Rhomboid intramembrane proteases are evolutionarily conserved proteins with numerous important biological functions, including growth factor secretion, regulation of mitochondrial dynamics, and membrane protein quality control (Fleig et al., 2012). Rhomboids are serine proteases with a Ser-His catalytic dyad (Wang et al., 2006), and they recognize their transmembrane substrates in a two-tier process. It is assumed that first a portion of the transmembrane domain of the substrate docks into an intramembrane interaction site of rhomboid within the plane of the lipid bilayer, upon which a linear segment of the substrate (possibly generated by local unfolding of the top of the substrate's transmembrane helix) interacts with the water-exposed active site (reviewed in Strisovsky, 2016a, Strisovsky, 2013).

To understand why peptidyl ketoamides are such efficient rhomboid inhibitors and to establish the basis for structure-guided design of their improved variants, we determined the co-crystal structures of GlpG with 9 and 10. The complexes were formed by soaking the inhibitors into apoenzyme crystals, and the structures were solved using diffraction data to 2.16 and 1.78 Å resolution, respectively, allowing detailed comparison of their binding modes. In both cases, the pentapeptide RVRHA binds the active site cavity as an extended β strand, virtually identically to the binding mode of Ac-RVRHA-cmk. We do observe weak electron density for the side chain of Arg in the P5 position, but its conformation in the final crystallographic models of the complexes of 9 and 10 differs, indicating some degree of flexibility, and it is probably influenced by crystal contacts. In addition, the P5 residue does not contribute significantly to the inhibition potency of 9 and is thus dispensable. In both inhibitors, the ketoamide warhead is covalently bonded via its proximal carbon to the side-chain oxygen of the catalytic S201, and it engages in a network of six hydrogen bonds in the active site. The tail substituents of 9 and 10 (RT9 and RT10) interact with the prime side of GlpG, buried in a cavity delimited by the side chains of amino acids F245, M247, and M249 from the L5 loop, W236 from TMD5, F153 and W157 from TMD2, and residues V204, M208, Y205, H254, H150, and N154. The NH group of the side chain of W236 seems to form a weak H-π bond with the phenyl ring of the tail of both compounds, and F245 engages in π…π stacking against the dimethylbenzyl in RT10.

> ERAGPVTWVMMIACVVVFIAMQILGDQEVMLWLAWPFDPTLKFEFWRYFTHALMHFSLMHILFNLLWWWYLGGAVEKRLGSGKLIVITLISALLSGYVQQKFSGPWFGGLSGVVYALMGYVWLRGERDPQSGIYLQRGLIIFALIWIVAGWFDLFGMSMANGAHIAGLAVGLAMAFVDSL> DADLDKQVNTAGAWPIATGGYYSQHNSPLAQINKSNVKNVKAAWSFSTGVLNGHEGAPLVIGDMMYVHSAFPNNTYALNLNDPGKIVWQHKPKQDASTKAVMCCDVVDRGLAYGAGQIVKKQANGHLLALDAKTGKINWEVEVCDPKVGSTLTQAPFVAKDTVLMGCSGAELGVRGAVNAFDLKTGELKWRAFATGSDDSVRLAKDFNSANPHYGQFGLGTKTWEGDAWKIGGGTNWGWYAYDPKLNLFYYGSGNPAPWNETMRPGDNKWTMTIWGRDLDTGMAKWGYQKTPHDEWDFAGVNQMVL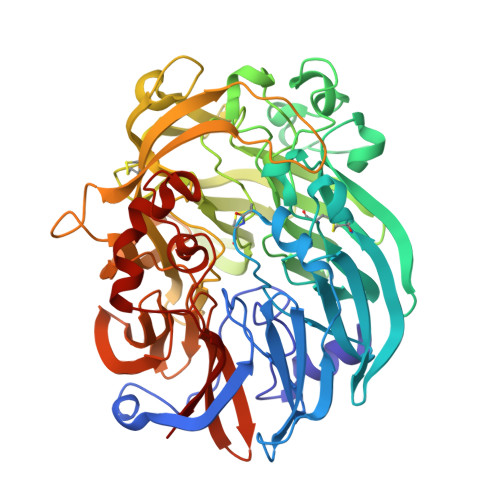TDQPVNGKMTPLLSHIDRNGILYTLNRENGNLIVAEKVDPAVNVFKKVDLKTGTPVRDPEFATRMDHKGTNICPSAMGFHNQGVDSYDPESRTLYAGLNHICMDWEPFMLPYRAGQFFVGATLAMYPGPNGPTKKEMGQIRAFDLTTGKAKWTKWEKFAAWGGTLYTKGGLVWYATLDGYLKALDNKDGKELWNFKMPSGGIGSPMTYSFKGKQYIGSMYGVGGWPGVGLVFDLTDPSAGLGAVGAFRELQNHTQMGGGLMVFSL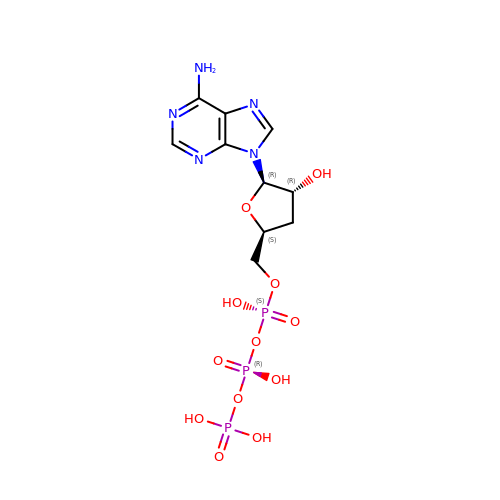3'-DEOXYADENOSINE-5'-TRIPHOSPHATE | C10 H16 N5 O12 P3 | NLIHPCYXRYQPSD-BAJZRUMYSA-N>MTSTNPVKDSYNKDAVFTYELIANPDADYSDQKLILKKEISYIKLNLGINQDNKNAPSYIFNLLDDNVYYGFYRDTQDMNRIENKYTYAFKKEAENFDNLQKFNATYEGQFWFSSIDTPNVPTVARAFLTYNNGRVDGEILAKHWNEKLFQITGFDNNPRKVEIFP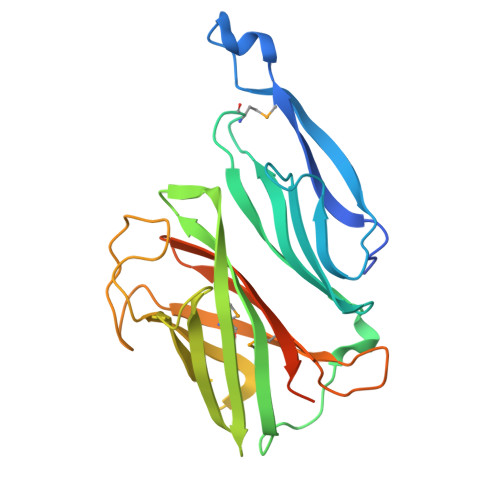TVEYLPNSGTRLTKGATSPHRFQMDLHFINSTNGEKNKYLVGQGSTEQYWGVLGMAAAQELALVPRGSSAHHHHHHHHHH[2x]>[2x]GPGSMAATIRYHEGDISAEDAARYKGAIAIDTETLGLVPRRDRLCVVQLSSGDGTADVIRIAAGQKQAPNLVHMLADPARQKIFHYGRFDIAVLFHTFGVTTTPVFCTKIASRLCRTYTDRHGLKDNLKEMLEVDISKAQQSSDWAAETLSPAQLEYAASDVLYLHALRDKLTARLIRDGRIEHADACFAFLPTRAKLDLLGWDETDIFAHS

The Agrobacterium tumefaciens genome contains two homologues of RNase D, Atu1151 (denoted At_RND, 30% similarity with full-length Ec_RND) and Atu4108 (denoted At_NrnC, 31% similarity with the N-terminal 184 residues of Ec_RND). At_RND contains an exonuclease domain and two HRDC domains, whereas At_NrnC contains a single DEDDy domain. At_NrnC forms an octameric hollow cylindrical structure, which allows dsDNA, ssDNA, and ssRNA to enter the central tunnel where the multiple active sites perform hydrolysis. This novel structural feature accounts for the high processivity of At_NrnC and its preference for longer dsDNA substrates despite the lack of HRDC domains.

The crystal structure of apo-At_NrnC was determined at 1.5 Å resolution and those of two forms of At_NrnC-Mn2+ were determined at 2.5 Å and 2.3 Å resolution. The apo and metal-bound structures were almost identical and only minor differences were observed. The final model of Atu4108 contained two protein molecules in the asymmetric unit. The At_NrnC protomer consisted of seven α helices and six β strands. The β-sheet region comprised all six β strands and extended from the surface to the central core. The remaining seven α helices and loops surrounded the above-mentioned strands and made contact with the other molecule of the asymmetric unit. The C-terminal loop extended into a pocket in the second molecule formed from the α3, α4, and α7 helices and the β6 strand. The α7 helix was slightly bent in the middle to better accommodate the C-terminal loop.>[2x]MLVEEEGRIRAMRAARSLGERTVTELILQHQNPQQLSSNLWAAVRARGCQFL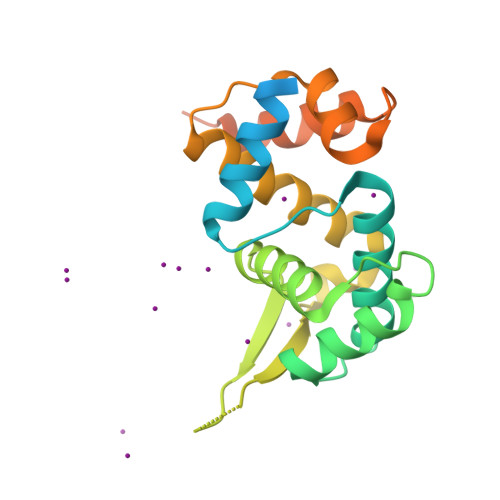GPAMQEEALKLVLLALEDGSALSRKVLVLFVVQRLEPRFPQASKTSIGHVVQLLYRASCFKVTKRDEDSSLMQLKEEFRTYEALRREHDSQIVQIAMEAGLRIAPDQWSSLLYGDQSHKSHMQSIIDKLQTPASFAQSVQELTIALQRTKHHHHHH BpsR is a member of the MarR family of bacterial transcriptional regulators. MarR proteins often repress genes involved in the response to organic compounds, environmental stresses, and virulence factors. They are obligate homodimers and many are responsive to ligand binding. Recently, we and others have shown that BpsR controls the growth of B. bronchiseptica by repressing genes involved in nicotinic acid (NA) degradation. BpsR repression is relieved by binding of 6-hydroxynicotinic acid (6HNA), allowing tight regulation of the pathway to control NA metabolism according to the needs and environment of the bacterium.

To elucidate the structural details of this regulation, we determined the structure of BpsR in complex with 6HNA. 6HNA-BpsR crystallized in the centered orthorhombic space group (C2221), with 6 chains in the asymmetric unit. Each dimer bound 2 molecules of 6HNA. The binding pockets are located at the dimer interface between helices α1, α2, α5 of one monomer and α1 of the opposing monomer, and are approximately 8 Å above the recognition helix of the HTH domain. The bound 6HNA is positioned between four amino acid residues extending from the α1 helix on both monomers. Residues Tyr15, His23, and Arg26 from one monomer and His32 from the other monomer each contribute to hydrogen bonding interactions with 6HNA. A comparison of the conformations of these residues shows that the side chain of Tyr15 shifts approximately 2 Å toward the 6HNA when compared to the unbound structure to H-bond with the 6-hydroxy group of the pyridine ring. The guanidinium moiety of Arg26 rotates approximately 5 Å away from the binding pocket, using its delta carbon as a hinge, to accommodate the entrance of 6HNA. A superimposition of the 6-HNA bound and apo BpsR structures reveals a conformational change within the dimer in which the wHtH motif of one monomer pivots away from the other resulting in a 7.3 Å increase in the distance between the α4 DNA recognition helices. This open conformation with an alteration to the inter-helical distance likely prevents them from inserting into consecutive DNA major grooves thus decreasing binding affinity.

>MPASQDKLDVPPGPYHFSEQVGHLLRRAYQRHVAIFQQTIPDSKLTAAQFVVLCALRDQGACSLVDVVKATAIDQATVRGVIERLKARKLLAVSHDPADRRKVLVTLTPDGRALVEEMVPFAEQITQSTFGGLNPAERVAIVYLLRKMSDADDLVGRQSDS[6x]Anion exchanger 3 (AE3) is pivotal in regulating intracellular pH across excitable tissues, yet its structural intricacies and functional dynamics remain underexplored compared to other anion exchangers. This study unveils the structural insights into human AE3, including the cryo-electron microscopy structures for AE3 transmembrane domains (TMD) and a chimera combining AE3 N-terminal domain (NTD) with AE2 TMD (hAE3NTD2TMD). Our analyzes reveal a substrate binding site, an NTD-TMD interlock mechanism, and a preference for an outward-facing conformation. Unlike AE2, which has more robust acid-loading capabilities, AE3’s structure, including a less stable inward-facing conformation due to missing key NTD-TMD interactions, contributes to its moderated pH-modulating activity and increased sensitivity to the inhibitor DIDS.

The structure of hAE3 in the presence of HCO3− and HCO3−/DIDS, and without HCO3− supplementation were determined with C2 symmetry, reaching overall resolutions of 2.7 Å, 2.7 Å, and 2.9 Å, respectively. In all three cryo-EM structures, hAE3 TMD consistently adopts an outward-facing conformation, demonstrating a high degree of structural conservation compared to human AE1 and AE2 in their respective outward-facing conformations. In the hAE3-DIDS structure, the cryo-EM density map of DIDS extends continuously to the sidechain of K842, indicating a covalent linking. Viewed from the extracellular side, DIDS is positioned near the outer vestibule’s exit/entrance atop the HCO3− anion, effectively obstructing the pathway between the substrate-binding site and the extracellular environment. Structural analysis of DIDS-contacting residues reveals that the core stilbene framework is encircled by hydrophobic residues such as L772/729, F726/835/1181, V773, and I831, which facilitate hydrophobic interactions stabilizing DIDS. Additionally, polar residues like T725, S1178, and E838 are near the stilbene’s isothiocyano groups. Interestingly, the residue K1173, a potential reactive site, appears unbonded with DIDS, as indicated by its separate density. In contrast, in the hAE3HCO3−/DIDS structure, the distance between the sulfonic acid groups of DIDS and the bicarbonate ion exceeds 5.4 Å, allowing for their simultaneous presence within the outer vestibule. Another distinguishing feature of AE3 is its heightened sensitivity to the pan-anion exchanger inhibitor DIDS relative to AE230. The increased vulnerability may stem from the predominant outward-facing conformation of AE3 under various tested pH and anion conditions, which renders its DIDS-binding site more accessible from the extracellular milieu.

>[2x]MANGVIPPPGGASPLPQVRVPLEEPPLSPDVEEEDDDLGKTLAVSRFGDLISKPPAWDPEKPSRSYSERDFEFHRHTSHHTHHPLSARLPPPHKLRRLPPTSARHTRRKRKKEKTSAPPSEGTPPIQEEGGAGVDEEEEEEEEEEGESEAEPVEPPHSGTPQKAKFSIGSDEDDSPGLPGRAAVTKPLPSVGPHTDKSPQHSSSSPSPRARASRLAGEKSRPWSPSASYDLRERLCPGSALGNPGGPEQQVPTDEAEAQMLGSADLDDMKSHRLEDNPGVRRHLVKKPSRTQGGRGSPSGLAPILRRKKKKKKLDRRPHEVFVELNELMLDRSQEPHWRETARWIKFEEDVEEETERWGKPHVASLSFRSLLELRRTIAHGAALLDLEQTTLPGIAHLVVETMIVSDQIRPEDRASVLRTLLLKHSHPNDDKDSGFFPRNPSSSSMNSVLGNHHPTPSHGPDGAVPTMADDLGEPAPLWPHDPDAKEKPLHMPGGDGHRGKSLKLLEKIPEDAEATVVLVGCVPFLEQPAAAFVRLNEAVLLESVLEVPVPVRFLFVMLGPSHTSTDYHELGRSIATLMSDKLFHEAAYQADDRQDLLSAISEFLDGSIVIPPSEVEGRDLLRSVAAFQRELLRKRREREQTKVEMTTRGGYTAPGKELSLELGGSEATPEDDPLLRTGSVFGGLVRDVRRRYPHYPSDLRDALHSQCVAAVLFIYFAALSPAITFGGLLGEKTEGLMGVSELIVSTAVLGVLFSLLGAQPLLVVGFSGPLLVFEEAFFKFCRAQDLEYLTGRVWVGLWLVVFVLALVAAEGSFLVRYISPFTQEIFAFLISLIFIYETFYKLYKVFTEHPLLPFYPPEGALEGSLDAGLEPNGSALPPTEGPPSPRNQPNTALLSLILMLGTFFIAFFLRKFRNSRFLGGKARRIIGDFGIPISILVMVLVDYSITDTYTQKLTVPTGLSVTSPDKRSWFIPPLGSARPFPPWMMVAAAVPALLVLILIFMETQITALIVSQKARRLLKGSGFHLDLLLIGSLGGLCGLFGLPWLTAATVRSVTHVNALTVMRTAIAPGDKPQIQEVREQRVTGVLIASLVGLSIVMGAVLRRIPLAVLFGIFLYMGVTSLSGIQLSQRLLLILMPAKHHPEQPYVTKVKTWRMHLFTCIQLGCIALLWVVKSTAASLAFPFLLLLTVPLRHCLLPRLFQDRELQALDSEDAEPNFDEDGQDEYNELHMPV>[8x]ANIQSFSFKNFNSPSFILQGDATVSSGKLQLTKVKENGIPTPSSLGRAFYSSPIQIYD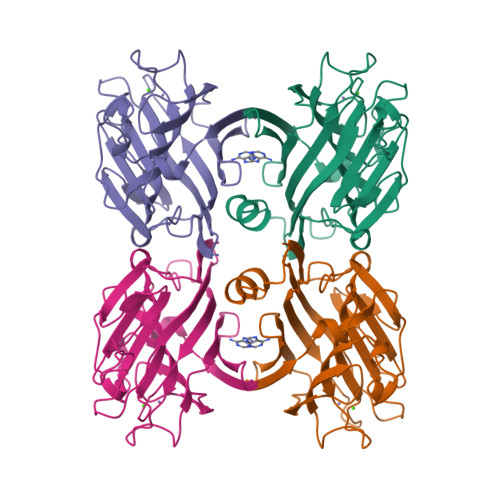KSTGAVASWATSFTVKISAPSKASFADGIAFALVPVGSEPRRNGGYLGVFDSDVYNNSAQTVAVEFDTLSNSGWDPSMKHIGIDVNSIKSIATVSWDLANGENAEILITYNAATSLLVASLVHPSRRTSYILSERVDITNELPEYVSVGFSATTGLSEGYIETHDVLSWSFASKLPDDSTAEPLDLASYLVRNVL(2R)-2-[{(E)-2-[({(2R,3R,4R,5S,6R)-3-(acetylamino)-4,5-bis(acetyloxy)-6-[(acetyloxy)methyl]tetrahydro-2H-pyran-2-yl}carbamothioyl)amino]ethenyl}(biphenyl-4-ylsulfonyl)amino]-3-methylbutanoic acid | C34 H42 N4 O12 S2 | 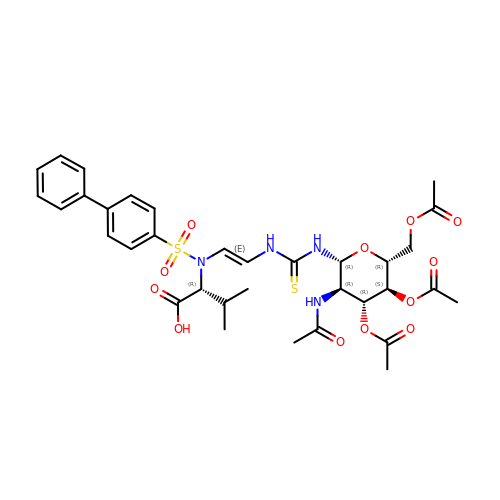NIEQAOCPXJWQAU-NPCCVVQBSA-N> GHHHIVK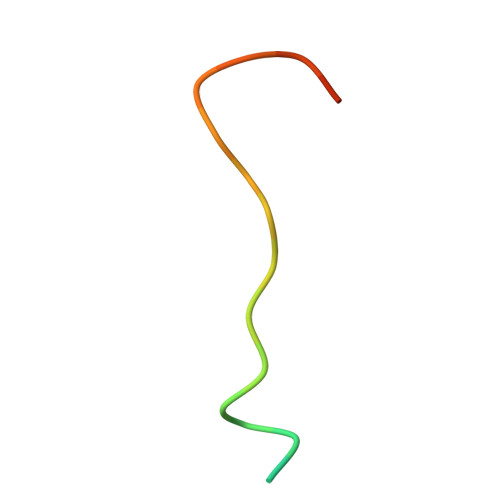FLLDFGVNVNAADSDG> ALEVDFKKLKQIKNRMKKTDWLFLNACVGVVEGDLAAIEAYKSSGGDIARQLTADEVRLLNRPSAFDVGYTLVHLAIRFQRQDMLAILLTEVSQQAAKCIPAMVCPELTEQIRREIAASLHQRKGDFACYFLTDLVTFTLPADI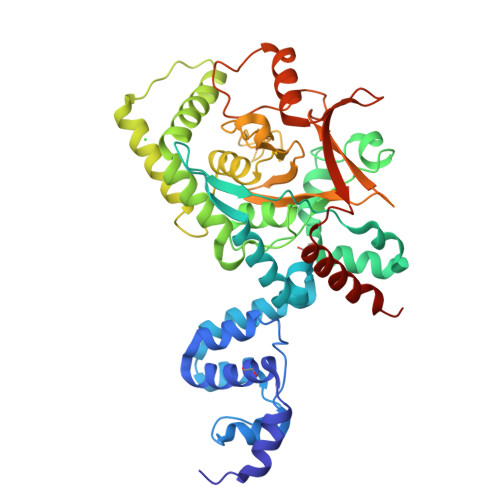EDLPPTVQEKLFDEVLDRDVQKELEEESPIINWSLELATRLDSRLYALWNRTAGDCLLDSVLQATWGIYDKDSVLRKALHDSLHDCSHWFYTRWKDWESWYSQSFGLHFSLREEQWQEDWAFILSLASQPGASLEQTHIFVLAHILRRPIIVYGVKYYKSFRGETLGYTRFQGVYLPLLWEQSFCWKSPIALGYTRGHFSALVAMENDGYGNRGAGANLNTDDDVTITFLPLVDSERKLLHVHFLSAQELGNEEQQEKLLREWLDCCVTEGGVLVAMQKSSRRRNHPLVTQMVEKWLDRYRQIRPCTSLS>MSVSAFNRRWAAVILEALTRHGVRHICIAPGSRSTPLTLAAAENSAFIHHTHFDERGLGHLALGLAKVSKQPVAVIVTSGTAVANLYPALIEAGLTGEKLILLTADRPPELIDCG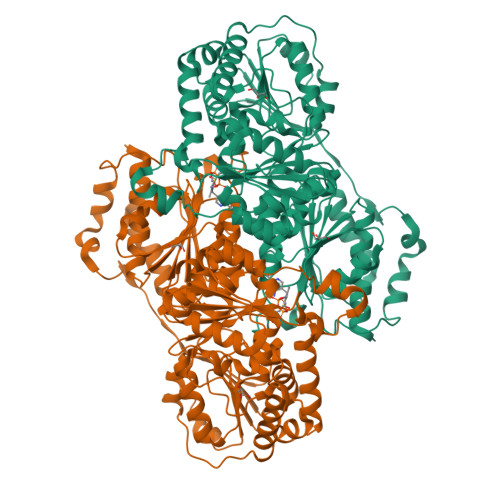ANQAIRQPGMFASHPTHSISLPRPTQDIPARWLVSTIDHALGTLHAGGVHINCPFAEPLYGEMDDTGLSWQQRLGDWWQDDKPWLREAPRLESEKQRDWFFWRQKRGVVVAGRMSAEEGKKVALWAQTLGWPLIGDVLSQTGQPLPCADLWLGNAKATSELQQAQIVVQLGSSLTGKRLLQWQASCEPEEYWIVDDIEGRLDPAHHRGRRLIANIADWLELHPAEKRQPWCVEIPRLAEQAMQAVIARRDAFGEAQLAHRICDYLPEQGQLFVGNSLVVRLIDALSQLPAGYPVYSNRGASGIDGLLSTAAGVQRASGKPTLAIVGDLSALYDLNALALLRQVSAPLVLIVVNNNGGQIFSLLPTPQSERERFYLMPQNVHFEHAAAMFELKYHRPQNWQELETAFADAWRTPTTTVIEMVVNDTDGAQTLQQLLAQVSHL[8x]>[2x]GPGNRKTKEIGEEPDPEKLEAFLEEKGGNALSHLGFLGDKRFFYSSDGNALIQFAKVGQRLVVLGDPSGREDSFPLVIKEFLHAADQKGYLVIFYQIEREDMALYHDFGYRFFKLGEEAIVDLDTFTISGKKRAGLRAIYNRFEREGYTFHVEQPPFSREFLNELRQVSDEWLGRKKEKGFSLG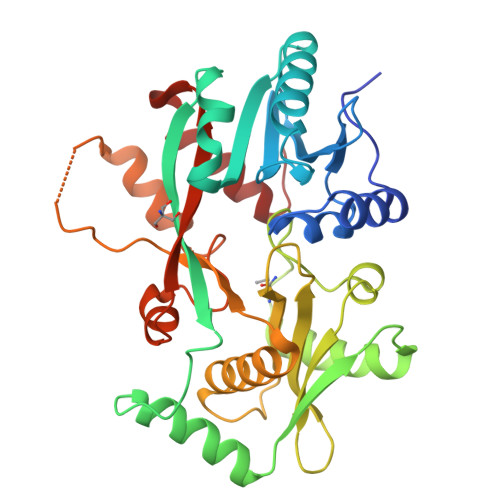FFQEDYLQKAPIAVLKSEEGEIVAFMNIMPMYREGEISIDLMRYSKKAPKGIMDALFIYLFQWGKEQGYTAFNMGMAPLSNVGTTFQSFWTERLAAVIFNNVSYMYSFSGLRSFKEKYKPVWRGKYLAYRKNRSLPVTMILVTRLIGRRTK Abiraterone | 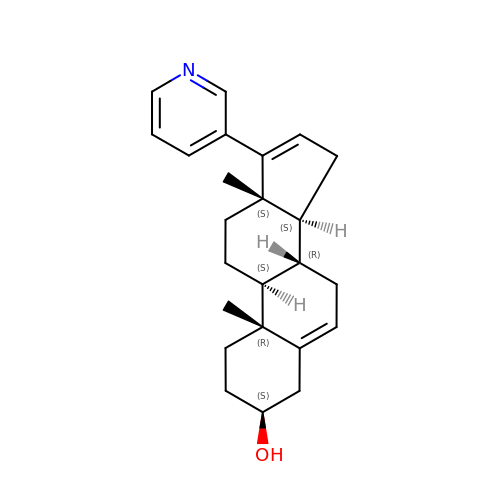C24 H31 N O | GZOSMCIZMLWJML-VJLLXTKPSA-N> HHHHHHIEGRGAYVLDDSDGLGREFDGIGAVSGGGATSRLLVNYPEPYRSEILDYLFKPNFGASLHILKVEIGGDGQTTDGTEPSHMHYELDENYFRGYEWWLMKEAKKRNPDIILMGLPWSFPGWLGKGFSWPYVNLQLTAYYVVRWILGAKHYHDLDIDYIGIWNERPFDANYIKELRKMLDYQGLQRVRIIASDNLWEPISSSLLLDQELWKVVDVIGAHYPGTYTVWNAKMSGKKLWSSEDFSTINSNVGAGCWSRILNQNYINGNMTSTIAWNLVASYYEELPYGRSGLMTAQEPWSGHYVVASPIWVSAHTTQFTQPGWYYLKTVGHLEKGGSYVALTDGLGNLTIIIETMSHQHSMCIRPYLPYYNVSHQLATFTLKGSLREIQELQVWYTKLGTPQQRLHFKQLDTLWLLDGSGSFTLELEEDEIFTLTTLTTGRKGSYPPPPSSKPFPTNYKDDFNVEYPLFSEAPNFADQTGVFEYYMNNEDREHRFTLRQVLNQRPITWAADASSTISVIGDHHWTNMTVQCDVYIETPRSGGVFIAGRVNKGGILIRSATGVFFWI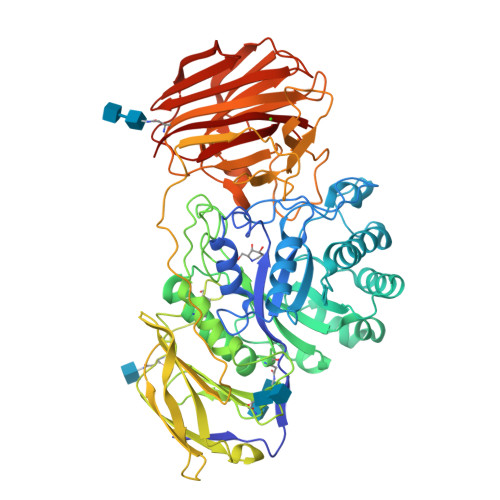FANGSYRVTADLGGWITYASGHADVTAKRWYTLTLGIKGYFAFGMLNGTILWKNVRVKYPGHGWAAIGTHTFEFAQFDNFRVEAAR> MLNQELELSLNMAFARAREHRHEF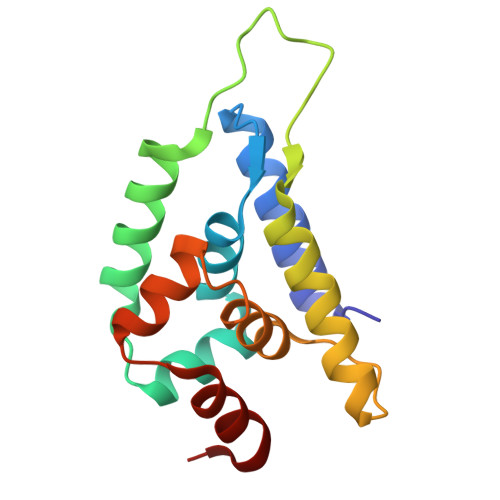MTVEHLLLALLSNPSAREALEACSVDLVALRQELEAFIEQTTPVLPASEEERDTQPTLSFQRVLQRAVFHVQSSGRNEVTGANVLVAIFSEQESQAAYLLRKHEVSRLDVVNFISHGT>MTITALPTGLYAEV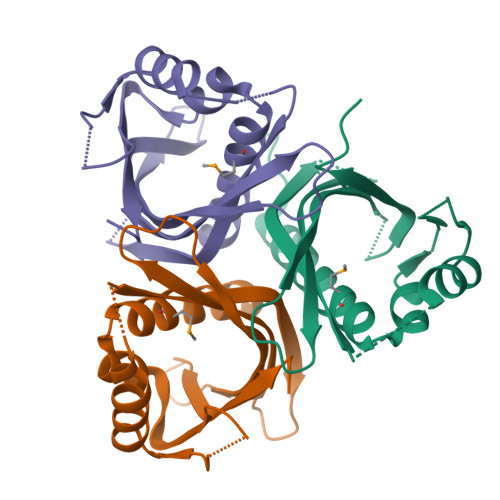LSFYGHQMQKLDGRDFAGYAATFTEDGEFRHSPSLPAAHTRAGITAVLEDFHRKFDARKIQRRHWFDHTALSQASDGSITATSYCLVLTVHADVKAPEFGPSCLVHDVLVRGADGELLLRSRHVTHDHVFPA[6x]> MLEQPYLDLAKKVLDEGHFKPDRTHTGTYSIFGHQMRFDLSKGFPLLTTKKVPFGLIKSELLWFLHGDTNIRFLLQHRNHIWDEWAFEKWVKSDEYHGPDMTDFGHRSQKDPEFAAVYHEEMAKFDDRVLHDDAFAAKYGDLGLVYGSQWRAWHTSKGD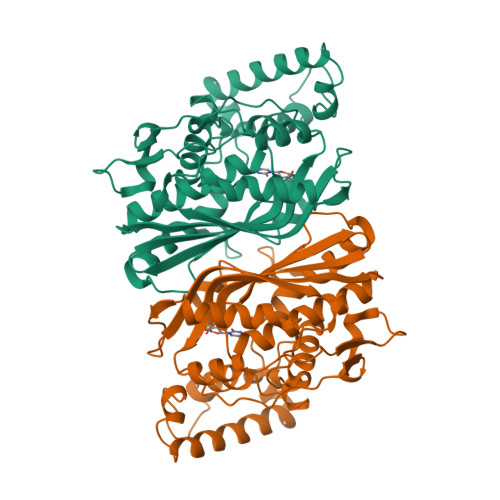TIDQLGDVIEQIKTHPYSRRLIVSAWNPEDVPTMALPPCHTLYQFYVNDGKLSLQLYQRSADIFLGVPFNIASYALLTHLVAHECGLEVGEFIHTFGDAHLFVNHLDQIKEQLSRTPRPAPTLQLNPDKHDIFDFDMKDIKLLNYDPYPAIKAPVAV Enzymes that catalyze disulfide bond formation in the periplasm of many Gram-negative bacteria are essential for virulence. This family of disulfide oxidoreductases, in particular the primary oxidase DsbA and its partner membrane-protein DsbB, co-operate to catalyze the oxidative folding of disulfide bond containing proteins, many of which are secreted or cell-surface virulence factors. Deletion of P. aeruginosa dsbA1 (that encodes PaDsbA1) elicits numerous effects in phenotypic assays including: inability to process elastase to a mature form; inability to export the Type 3 Secretion System (T3SS), and toxins ExoU or ExoT; impaired ability to survive intracellularly in HeLa cells; loss of twitching motility; and reduced alkaline phosphatase and lipase activity. Consequently PaDsbA1 is a highly significant control point affecting the function of many downstream virulence effector molecules and as such is a potential target for inhibitor development. As with other DsbA enzymes, the catalytic surface of PaDsbA1 is composed of a CPHC active site, and three neighbouring surface loops that determine redox character as well as the nature of interactions with substrates and the partner protein DsbB.

For all crystallization experiments we used the E82I variant of PaDsbA1. Crystal soaking experiments yielded a 1.45 Å resolution co-crystal structure of PaDsbA1-E82I in complex with Fragment 1 with an Rfactor/Rfree of 13.6%/16.3% respectively. In both the X-ray structure and the HADDOCK models of the complex, Fragment 1 is positioned at an interface between the thioredoxin (TRX) and helical domains of PaDsbA1, on the non-catalytic face of the enzyme. Fragment 1 bound to PaDsbA1 at the end of this groove adjacent to helix H6. The amino-triazole ring of Fragment 1 binds into a pocket that is formed by residues Tyr148, Ser22 and Glu28, where it is sandwiched between the surface formed by helix H6, the B2 sheet and B1-B2 connecting loop The ortho-methylbenzene group is positioned close to the interface of H6 and H2 of the helical domain. In the crystal structure however, the majority of observable contacts between PaDsbA1 and Fragment 1 are to this amino-triazole group for which the electron density map is sharply resolved. Specifically Fragment 1 is coordinated by two side-chain mediated hydrogen bonds between the amino substituent of the triazole ring and residues Glu28 (2.99 Å) and Tyr148 (2.92 Å). Additional stabilization is provided by a π-stacking interaction between the triazole ring and amide bond of Val21 –Ser22 (3.55 Å from centroid to Ser22 Cα). Electron density for the ortho-methylbenzene group is less well defined in the X-ray structure presumably the result of a degree of flexibility. The crystal structure of PaDsbA1 undergoes very minor conformational changes upon fragment binding.

> SNADDYTAGKEYVELSSPVPVSQPGKIEVVELFWYGCPHCYAFEPTIVPWSEKLPADVHFVRLPALFGGIWNVHGQMFLTLISMGVEHDVHNAVFEAIHKEHKKLATPEEMADFLAGKGVDKEKFLSTYNSFAIKGQMEKAKKLAMAYQVTGVPTMVVNGKYRFDIGSAGGPEETLKLADYLIEKERAAAKK> HMQEAERASASDFKNHQLPLARIKKIMKADEDV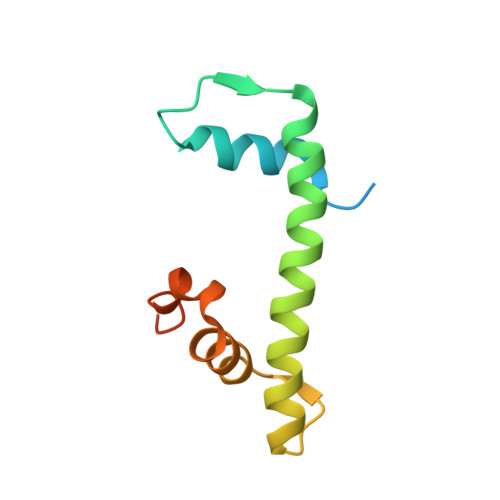RMISAEAPVLFAKACELFILELTIRSWLHAEENKRRTLQRNDVAAAIARTDVFDFLVDIVPREEAKEEPGS>STTEVVMENVTAFWEEGFGELFEKAKQNNNNRKTSNGDDSLSFSNFSLLGTPVLKDINFKIERGQ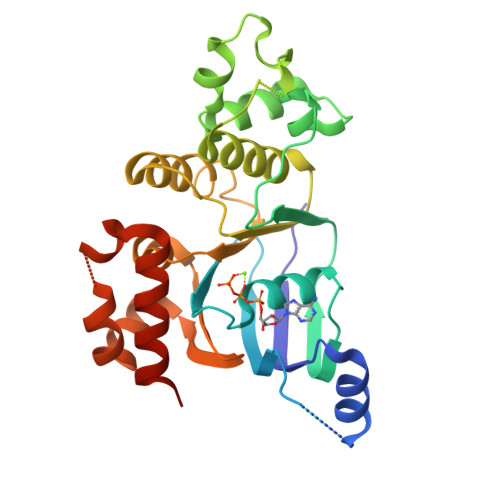LLAVAGSTGAGKTSLLMMIMGELEPSEGKIKHSGRISFCSQNSWIMPGTIKENIIGVSYDEYRYRSVIKACQLEEDISKFAEKDNIVLGEGGITLSGGQRARISLARAVYKDADLYLLDSPFGYLDVLTEKEIFESCVCKLMANKTRILVTSKMEHLKKADKILILHEGSSYFYGTFSELQNLRPDFSSKLMGCDSFDQFSAERRNSILTETLHRFSLEGDAPVS[2x]> NTIDEGLYSRQLYVLGHEAMKQMSQSNVLIIGCKGLGVEIAKNVCLAGVKSVTLYDPQPTRIEDLSSQYFLTEDDIGVPRAKVTVSKLAELNQYVPVSVVDELSTEYLKNFKCVVVTETSLTKQLEINDFTHKNHIAYIAADSRGLFGSIFCDFGENFICTDTDGNEPLTGMIASITDDGVVTMLEETRHGLENGDFVKFTEVKGMPGLNDGTPRKVEVKGPYTFSIGSVKDLGSAGYNGVFTQVKVPTKISFKSLRESLKDPEYVYPDFGKM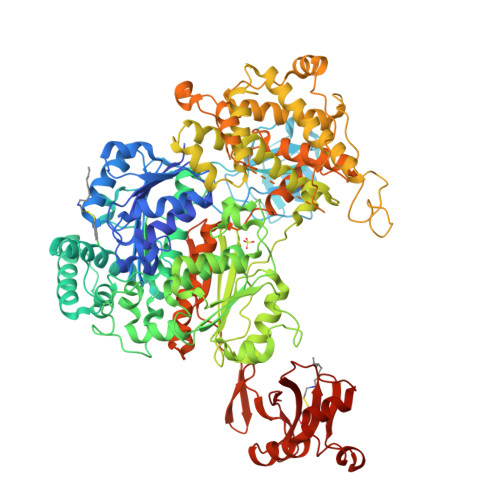MRPPQYHIAFQALSAFADAHEGSLPRPRNDIDAAEFFEFCKKIASTLQFDVELDEKLIKEISYQARGDLVAMSAFLGGAVAQEVLKATTSKFYPLKQYFYFDSLESLPSSVTISEETCKPRGCRYDGQIAVFGSEFQEKIASLSTFLVGAGAIGCEMLKNWAMMGVATGESGHISVTDMDSIEKSNLNRQFLFRPRDVGKLKSECASTAVSIMNPSLTGKITSYQERVGPESEGIFGDEFFEKLSLVTNALDNVEARMYVDRRCVFFEKPLLESGTLGTKGNTQVVVPHLTESYGSSQDPPEKSFPIATLKNFPNRIEHTIAWARDLFEGLFKQPIDNVNMYLSSPNFLETSLKTSSNPREVLENIRDYLVTEKPLSFEECIMWARLQFDKFFNNNIQQLLFNFPKDSVTSTGQPFWSGPKRAPTPLSFDIHNREHFDFIVAAASLYAFNYGLKSETDPAIYERVLAGYNPPPFAPKSGIKIQVNENEEAPETAANKDKQELKSIADSLPPPSSLVGFRLTPAEFEKDDDSNHHIDFITAASNLRAMNYDITPADRFKTKFVAGKIVPAMCTSTAVVSGLVCLELVKLVDGKKKIEEYKNGFFNLAIGLFTFSDPIASPKMKVNGKEIDKIWDRYNLPDCTLQELIDYFQKEEGLEVTMLSSGVSLLYANFQPPKKLAERLPLKISELVEQITKKKLEPFRKHLVLEICCDDANGEDVEVPFICIKL>MKEQLYTGLTEKEANQMQALLLSNDVNVSKEMDKSGNMTLSVAAADFVRAITILNNNGFPKKKFADIEVIFPPSQLVASPSQENAKINYLKEQDIERLLSKIPGVIDCSVSLNVNNNESQPSSAAVLVISSPEVNLAPSVIQIKNLVKNSVDDLKLENISVVIKSSSG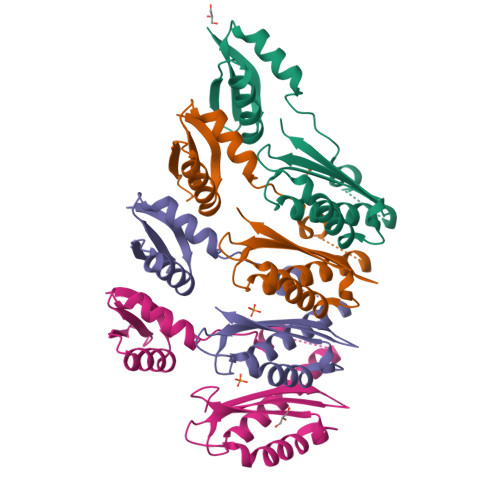QDG[4x]>[2x]MKMKLAVLPGDGIG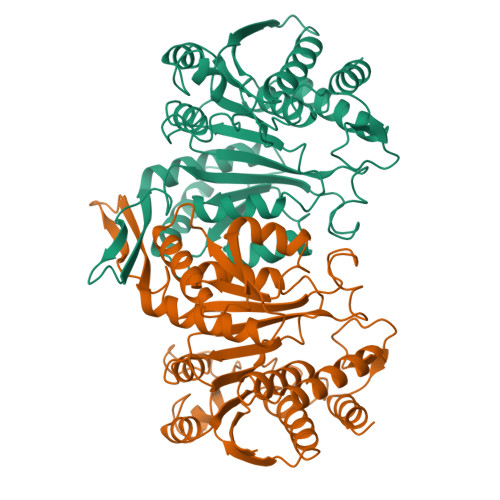PEVMDAAIRVLKTVLDNDGHEAVFENALIGGAAIDEAGTPLPEETLDICRRSDAILLGAVGGPKWDHNPASLRPEKGLLGLRKEMGLFANLRPVKAYATLLNASPLKRERVENVDLVIVRELTGGLYFGRPSERRGPGENEVVDTLAYTREEIERIIEKAFQLAQIRRKKLASVDKANVLESSRMWREIAEETAKKYPDVELSHMLVDSTSMQLIANPGQFDVIVTENMFGDILSDEASVITGSLGMLPSASLRSDRFGMYEPVHGSAPDIAGQGKANPLGTVLSAALMLRYSFGLEKEAAAIEKAVDDVLQDGYCTGDLQVANGKVVSTIELTDRLIEKLNNSAARPRIFQ> ADEPVWRSEQAIGAIAASQEDGVFVASGSCLDQLDYSLEHSLSRLYRDQAGNCTEPVSLAPPARPRPGSSFSKLLLPYREGAAGLGGLLLTGWTFDRGACEVRPLGNLSRNSLRNGTEVVSCHPQGSTAGVVYRAGRNNRWYLAVAATYVLPEPETASRCNPAASDHDTAIALKDTEGRSLATQELGRLKLCEGAGSLHFVDAFLWNGSIYFPYYPYNYTSGAATGWPSMARIAQSTEVLFQGQASLDCGHGHPDGRRLLLSSSLVEALDVWAGVFSAAAGEGQERRSPTTTALCLFRMSEIQARAKRVSWDFKTAESHCKEGDQPERVQPIASSTLIHSDLTSVYGTVVMNRTVLFLGTGDGQLLKVILGENLTSNCPEVIYEIKEETPVFYKLVPDPVKNIYIYLTAGKEVRRIRVANCNKHKSCSECLTATDPHCGWCHSLQRCTFQGDCVHSENLENWLDISSGAKKCPKIQIIRSSKEKTTVTMVGSFSPRHSKCMVKNVDSSRELCQNKSQPNRTCTCSIPTRATYKDVSVVNVMFSFGSWNLSDRFNFTNCSSLKECPACVETGCAWCKSARRCIHPFTACDPSDYERNQEQCPVAVEKTSGGGRPKENKGNRTNQALQVFYIKSIEPQKVSTLGKSNVIVTGANFTRASNITMILKGTSTCDKDVIQVSHVLNDTHMKFSLPSSRKEMKDVCIQFDGGNCSSVGSLSYIALPHCSLIFPATTWISGGQ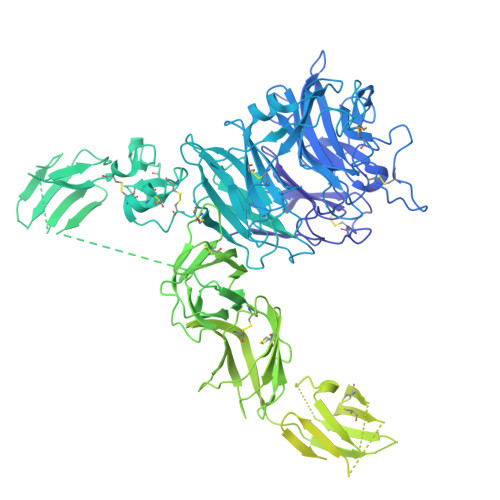NITMMGRNFDVIDNLIISHELKGNINVSEYCVATYCGFLAPSLKSSKVRTNVTVKLRVQDTYLDCGTLQYREDPRFTGYRVESEVDTELEVKIQKENDNFNISKKDIEITLFHGENGQLNCSFENITRNQDLTTILCKIKGIKTASTIANSSKKVRVKLGNLELYVEQESVPSTWYFLIVLPVLLVIVIFAAVGVTRHKSKELSRKQSQQLELLESELRKEIRDGFAELQMDKLDVVDSFGTVPFLDYKHFALRTFFPESGGFTHIFTEDMHNRDANDKNESLTALDALICNKSFLVTVIHTLEKQKNFSVKDRCLFASFLTIALQTKLVYLTSILEVLTRDLMEQCSNMQPKLMLRRTESVVEKLLTNWMSVCLSGFLRETVGEPFYLLVTTLNQKINKGPVDVITCKALYTLNEDWLLWQVPEFSTVALNVVFEKIPENESADVCRNISVNVLDCDTIGQAKEKIFQAFLSKNGSPYGLQLNEIGLELQMGTRQKELLDIDSSSVILEDGITKLNTIGHYEISNGSTIKVFKKIANFTSDVEYSDDHCHLILPDSEAFQDVQGKRHRGKHKFKVKEMYLTKLLSTKVAIHSVLEKLFRSIWSLPNSRAPFAIKYFFDFLDAQAENKKITDPDVVHIWKTNSLPLRFWVNILKNPQFVFDIKKTPHIDGCLSVIAQAFMDAFSLTEQQLGKEAPTNKLLYAKDIPTYKEEVKSYYKAIRDLPPLSSSEMEEFLTQESKKHENEFNEEVALTEIYKYIVKYFDEILNKLERERGLEEAQKQLLHVKVLFDEKKKCKWMGTSSGLEVLFQ> EEMKKGHLERECMEETCSYEEAREVFEDSDKTNEFWNKYKDGDQCETSPCQ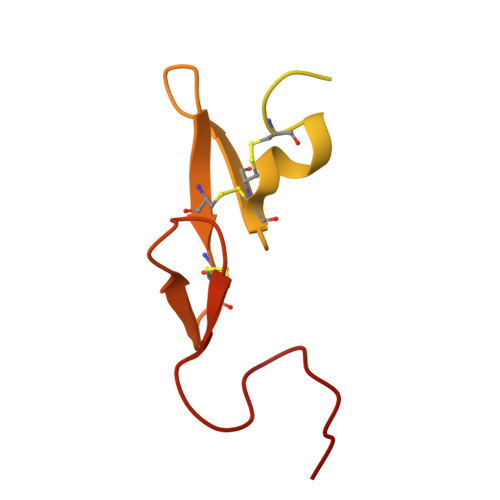NQGKCKDGLGEYTCTCLEGFEGKNCELFTRKLCSLDNGDCDQFCHEEQNSVVCSCARGYTLADNGKACIPTGPYPCGKQTLER(2S)-1-(4-{[2-(2-aminopyrimidin-5-yl)-7-methyl-4-(morpholin-4-yl)thieno[3,2-d]pyrimidin-6-yl]methyl}piperazin-1-yl)-2-hydroxypropan-1-one 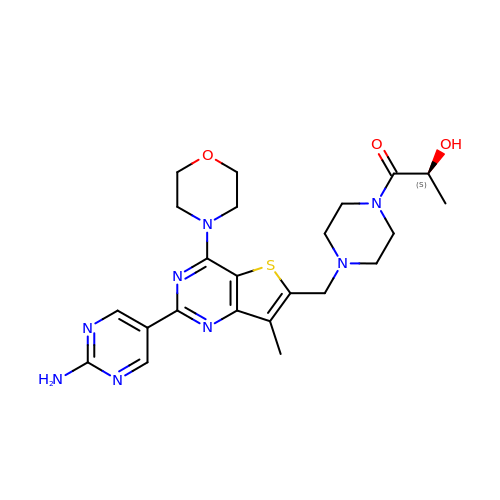| C23 H30 N8 O3 S | YOVVNQKCSKSHKT-HNNXBMFYSA-N> GSSVVVDTNGQPVSNGADAYYLVPVSHGHAGLALAKIGNEAEPRAVVLDPHHRPGLPVRFES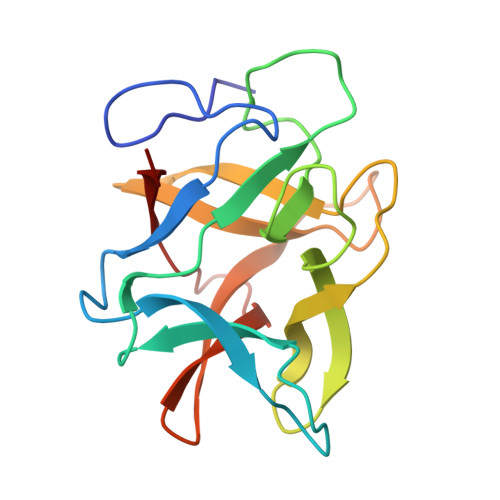PLFINIIKESYFLNIKFGPSSSDSGVWDVIQQDPIGLAVKVTDTKSLLGPFKVEKEGEGYKIVYYPERGQTGLDIGLVHRNDKYYLAVKDGEPCVFKIRKAT>[4x]MVRRTKEEAQETRAQIIEAAERAFYKRGVARTTLADIAELAGVTRGAIYWHFNNKAELVQALLDSLAETHDHLARASESEDEVDPLGCMRKL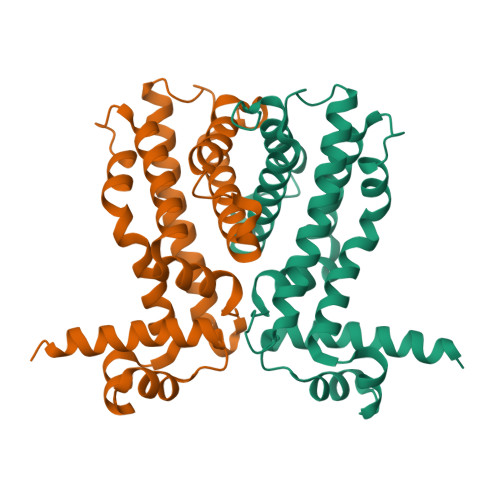LLQVFNELVLDARTRRINEILHHKCEFTDDMCEIRQQRQSAVLDCHKGITLALANAVRRGQLPGELDAERAAVAMFAYVDGLIRRWLLLPDSVDLLGDVEKWVDTGLDMLRLSPALRK>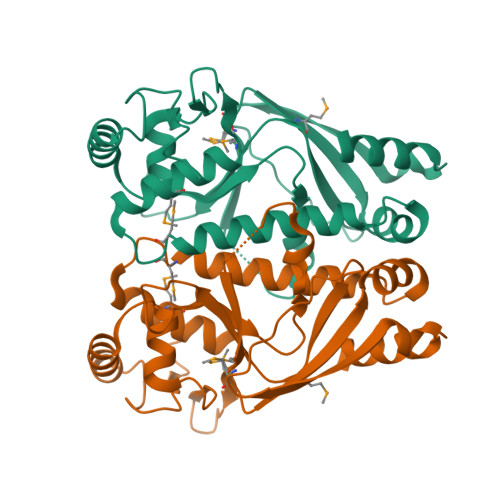 MHHHHHHMPEKLDTVLGYLKEFPDYYKYVTKKTYTLNEKIIFEDEKAKSIFFIVEGYAAVELEDNLRKTNYISIFVLPYNVLGIDAFSSYPKKKHSITVMSESLMLYKIDADFLLNILSIKPDVNDFLLTSIADVFARHYALLGMIAKTPKERIYMALENLAVEMGTEDEERNEIVLPNFINQSVLARYCRTTQPNISNLLTELVEEEFLINKKSPYRIDKDSLDI Rad2/XPG belongs to the flap endonuclease family that encompasses various structure-specific nucleases involved in nucleic acid processing. The unique feature of Rad2/XPG is the recognition of DNA bubbles that comprise a stretch of unpaired bases flanked by double-stranded regions and correspond to the DNA in the NER pre-incision complex. We report four structures of the Rad2 catalytic core solved in four different space groups, three of which represent the productive substrate binding mode and reveal that the protein recognizes a single 5′ nucleotide of the single-stranded portion of the DNA and a 3′ phosphate group of the ss/dsDNA junction. The two critical regions for substrate binding are the H2TH module with a Rad2-specific α-helix 12b and the hydrophobic wedge that binds the first base pair of the double-stranded portion of the DNA.

The structure of complex III was solved at 2.4 Å resolution. It comprised two Rad2-ΔSC molecules bound to a 15-mer DNA duplex with 1 nt single-stranded overhangs in all four ends of the DNA strands. Two copies of complex III were present in the asymmetric unit of its crystals. The productive complexes II–IV have the same overall architecture. In our structures, including complex IV in which the DNA had the longest overhangs (4 nt), we did not observe electron densities for the single-stranded regions of the DNA, except for the single nucleotide in the cleaved (5′ flap) strand that is visible in complexes III and IV. The phosphate group on the 3′ side of this single nucleotide is stabilized by van der Waals interactions with Tyr36 (from N region). For the non-cleaved (3′ flap) DNA strand, in one protein molecule of complex II and three protein molecules of complex III, we observed the electron density for the phosphate group of the ss/dsDNA junction. Several charged residues line a pocket located close to this phosphate: Arg60, Arg61 (both from the N region), His830 and Glu831 (from I region). All eight independently determined protein structures in complexes II–IV are essentially identical, with pairwise root-mean-square deviations (rmsds) between 0.5 and 0.8 Å over 273 to 285 C-α atoms. When all of the protein subunits from the productive complexes II–IV are compared, the DNA superimposes very well at the H2TH module, but its trajectory differs significantly in other regions, particularly around the hydrophobic wedge.

>GVHSFWDIAGPTARPVRLESLEDKRMAVDASIWIYQFLKAVRDQEGNAVKNSHITGFFRRICKLLYFGIRPVFVFDGGVPVLKRETIRQRKERRQGKRESAKSTARKLLANTTLSTSAERNVAENAFVEDELFEQQMKDKRDSDEVTMDMIKEVQELLSRFGIPYITAPMEAEAQCAELLQLNLVDGIITDDSDVFLFGGTKIYKNMFHEKNYVEFYDAESILKLLGLDRKNMIELAQLLGSDYTNGLKGMGPVSSIEVIAEFGNLKNFKDWYNNGQFDKRKQETENKFEKDLRKKLVNNEIILDDDFPSVMVYDAYMRPEVDHDTTPFVWGVPDLDMLRSFMKTQLGWPHEKSDEILIPLIRDV[4x]>MHHHHHHMIVRRATYEDLSQLAVLFDEYRQFYGASSNLEESHHFLKQRFENKESVFFIHIKDEKITGFVLLYLGFSSVACSTYYILDDVYVTPLFRRQGSAKQLIDTAILFAKQENALRISLETQSNNHESHRLFEKMGFIRDSEFQTFHCFLK[2x]

Here we have uncovered a GNAT-family acetyltransferase conserved in A. baumannii that is responsible for the acetylation of 1,3-DAP in A. baumannii in vivo and in vitro and renamed accordingly as Dpa for diamino-propane acetyltransferase. The crystal structure of Dpa reveals topological and functional differences from other bacterial polyamine acetyltransferases, adopting a β-swapped quaternary arrangement similar to that of eukaryotic polyamine acetyltransferases with a central size exclusion channel that sieves through the cellular polyamine pool. In this study, we have found a downstream regulatory element in this pathway: the polyamine acetyltransferase Dpa that specifically acetylates 1,3-DAP in A. baumannii to control the effective levels of the metabolite. The structure of Dpa revealed a dimeric architecture with a conserved acCoA and an acidic polyamine binding site formed at the dimer interface that shares properties with other polyamine acetyltransferases.

To gain insights into the catalytic mechanism of Dpa, we used a catalytically impaired version of the enzyme carrying Y128F mutation that allowed us to determine the structure of Dpa bound to 1,3-DAP and acCoA. The crystals of DpaY128F grown in the presence of acCoA were soaked between 30 s and 1 min with 1,3-DAP before vitrification in liquid N2. The compromised activity of DpaY128F allowed us to observe the post-catalysis state of the reaction with Ac-1,3-DAP bound to one of the two DpaY128F of the dimer. The other monomer of DpaY128F was bound to 1,3-DAP that was oriented slightly differently in the active site. Binding of the polyamine pre- or post-catalysis did not introduce major structural rearrangements. Interestingly, the orientation of 1,3-DAP in the active site of Dpa observed in the crystal structure was similar to that observed in mouse polyamine acetyltransferase SSAT14, suggesting that these subfamilies are functionally related. Two densities corresponding to metal ions occupied symmetrical positions at the dimer interface and coordinate D80 and D81, damping the negative charges of the active site. These ions hold together a network of water molecules that connected and accommodated the polyamine substrate. At the other end of the active site, 1,3-DAP is stabilized by contacts to E116 of one subunit and F139 of the other, both located at the narrow entrance of the β-swap channel, together with α1 Y25 and V71 of the β3-β4 turn. This architecture defines the pocket that accommodates the substrate and likely provides specificity to the enzyme.>[2x]MGSDKIHHHHHHE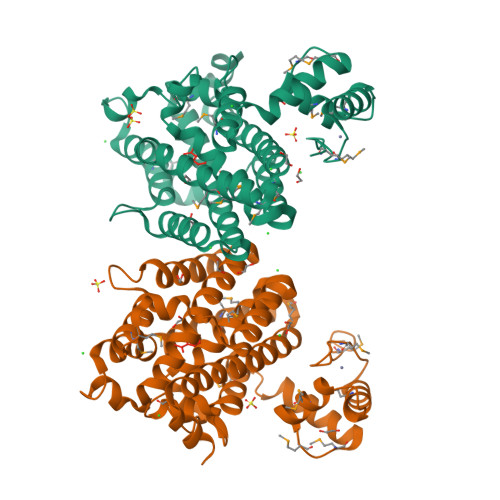NLYFQGMPLCPSCEMKFNSWEDLAKHMDLIANTNSDKSHVMWLNRNISMKRMEVNELANALERFFSTPNSLSMWIRTRFIERFYGDNPHPFIVAMQNPTKGVLLGYVIEHQHFLKNWVKVLSSIVFKTDKDDVLQYELENISVEFIGYNGRPAHYELLLRMGEALGMPREKILSTQPLPSTQSAIKTWRKIAESKTWLETMASMHSLELVADRSLVKYGAKLPYFNPEILSSDEYPQAVKDFLREGYEADVSHAGEALEMVEKYTEEMEMKEQVQITVLKSFDAFSKYLLARLERGFEIEPSLLKRVIK> G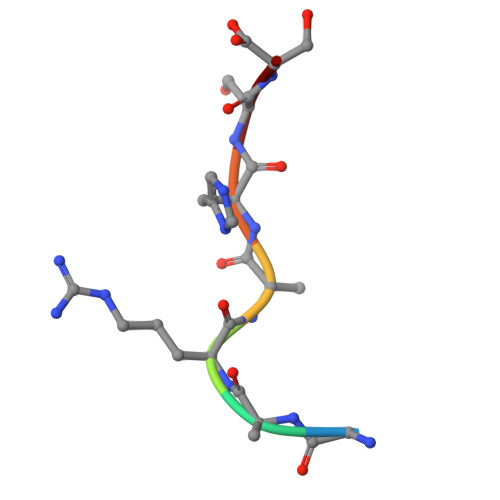ARAHSS> ETGEEPPRFIKEPKDQIGVSGGVASFVCQATGDPKPRVTWNKKGKKVNSQRFETIEFDESAGAVLRIQPLRTPRDENVYECVAQNSVGEITVHAKLTVLREDQLPSGFPNIDMGPQLKVVERTR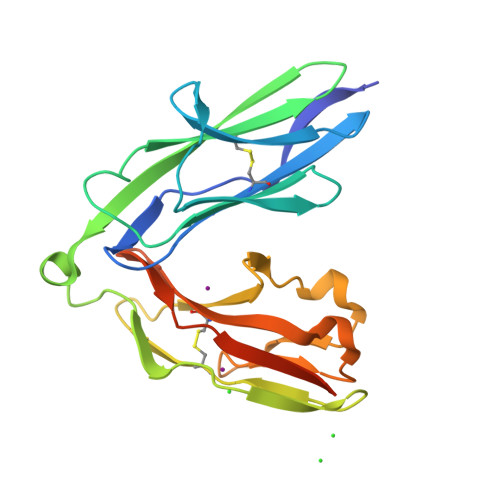TATMLCAASGNPDPEITWFKDFLPVDPSASNGRIKQLRSGALQIESSEETDQGKYECVATNSAGVRYSSPANLYVRVRRVAGTKHHHHHH>MAKQLQARRLDGIDYNPWVEFVKLASEHDVVNLGQGFPDFPPPDFAVEAFQHAVSGDFMLNQYTKTFGYPPLTKILASFFGELLGQEIDPLRNVLVTVGGYGALFTAFQALVDEGDEVIIIEPFFDCYEPMTMMAGGRPVFVSLKPGPIQNGELGSSSNWQLDPMELAGKFTSRTKALVLNTPNNPLGKVFSREELELVASLCQQHDVVCITDEVYQWMVYDGHQHISIASLPGMWERTLTIGSAGKTFSATGWKVGWVLGPDHIMKHLRTVHQNSVFHCPTQSQAAVAESFEREQLLFRQPSSY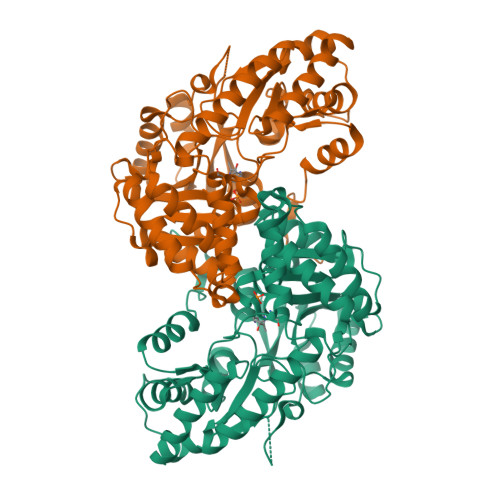FVQFPQAMQRCRDHMIRSLQSVGLKPIIPQGSYFLITDISDFKRKMPDLPGAVDEPYDRRFVKWMIKNKGLVAIPVSIFYSVPHQKHFDHYIRFCFVKDEATLQAMDEKLRKWKVEL[2x]>[2x]MSIEKIWAREILDSRGNPTVEVDLYTAKGLFRAAVPSGASTGIYEALELRDGDKQRYLGKGVLKAVDHINSTIAPALISSGLSVVEQEKLDNLMLELDGTENKSKFGANAILGVSLAVCKAGAAERELPLYRH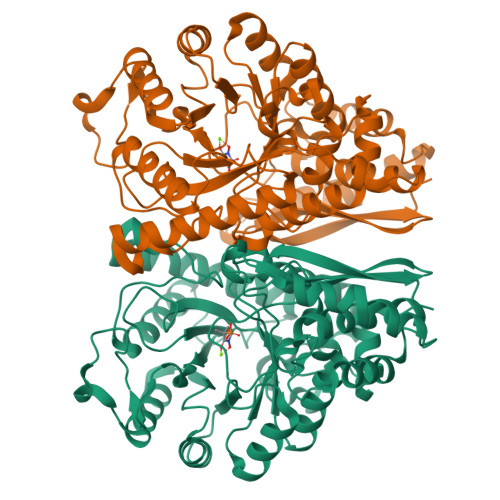IAQLAGNSDLILPVPAFNVINGGSHAGNKLAMQEFMILPVGAESFRDAMRLGAEVYHTLKGVIKDKYGKDATNVGDEGGFAPNILENSEALELVKEAIDKAGYTEKIVIGMDVAASEFYRDGKYDLDFKSPTDPSRYITGDQLGALYQDFVRDYPVVSIEDPFDQDDWAAWSKFTANVGIQIVGDDLTVTNPKRIERAVEEKACNCLLLKVNQIGSVTEAIQACKLAQENGWGVMVSHRSGETEDTFIADLVVGLCTGQIKTGAPCRSERLAKYNQLMRIEEELGDEARFAGHNFRNPSVLHHHHHH>GSHMASSCAVQVKLELGHRAQVRKKPTVEGFTHDWMVFVRGPEHSNIQHFVEKVVFHLHESFPRPKRVCKDPPYKVEESGYAGFILPIEVYFKNKEEPRKVRFDYDLFLHLEGHPPVNHLRCEKLTFNNPTED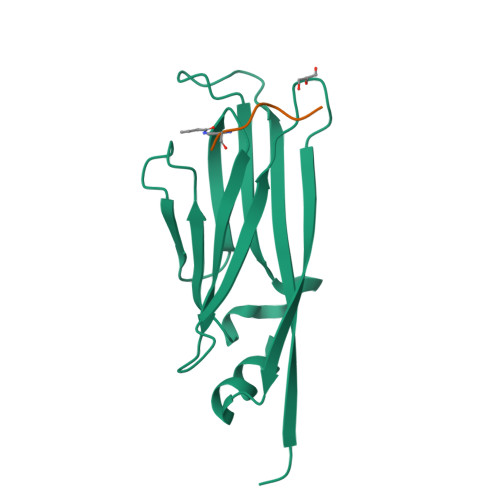FRRKLLKA[2x];>[2x]ARTKQTARXSTGGKAPRKQ>MSSVQSSQTQKNDDAEVFDALIVGAGFNGIYQLHRLRQEGFKVRLFEAGADMGGIWYWNCYPGARVDSHIPIYEFSIEELWRDWNWTERFPAWDELRRYFHYVDKKLDLSRDIRFGMRVSAAEFDEARDQWVIRTTDGTVVRARFFILCTGFASKPYIPNYKGLESFAGESFHTGLWPQEGASFTGKRVGVVGTGASGVQVVQEASKDAAHLTVFQRTPILALPMQQRKLDVETQQRMKADYPEIFRIRRETFGGFDILRDERSALEVPPEERCALYEKLWQKGGF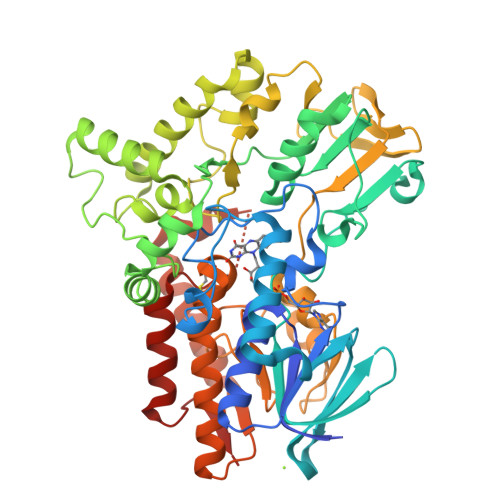HYWIGGFSDILTNEEANRTMYDFWRDKTRARIKNPALADKLAPMEPPHPFGVKRPSLEQWYYEAFNQDNVSLVDVREMPIVEIVPEGVLTSDGLVELDMLVLATGFDAVTGGLTQIDIHGTGGITLKEKWTEGARTYLGFATSGFPNMLFLYGPQSPSGFCNGPTCAEMQGEWVVDCLKHMRENNKGRIEATAQAEEEWAQLLNSIAGMTLFPRADSWYMGANIPGKPRQLLNFPGVPIYMDQCNTAAAKDYEGFVLD[2x]> GPLGSGRPMLSTDNFKKIKLRDISLEDAIKASNYEEINNK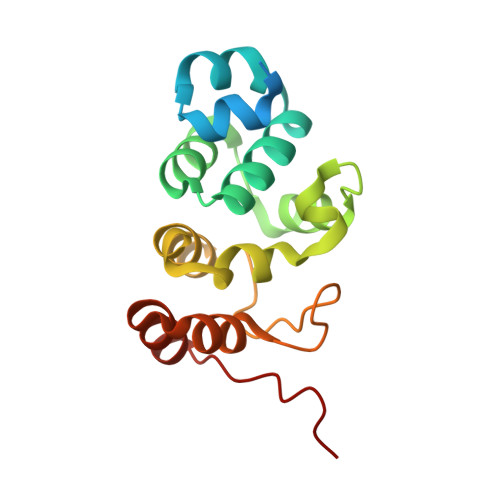VTDKKMAHQALAYSLGNKKADIALYLLSKFNFTKQDVAEMEKMKNNRYCNLYDVEYLLSKDGANYKVLEYFINNGLVDVNKKFQKVNSGDTMLDNAMKSKDSKMIDFLLKNGAILGKRFEI> YNRLCIKPRDWIDECDSNEGGERAYFRNGKGGCDSFWICPEDH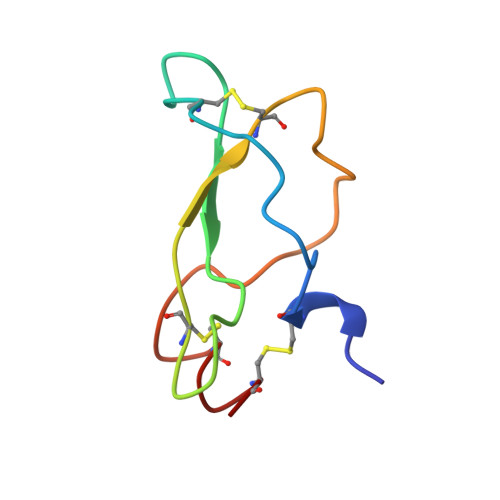TGADYYSSYRDCFNACI2-(1,3-dimethoxypropan-2-yl)-1,2,3,4-tetrahydroisoquinolin-8-amine | C14 H22 N2 O2 | 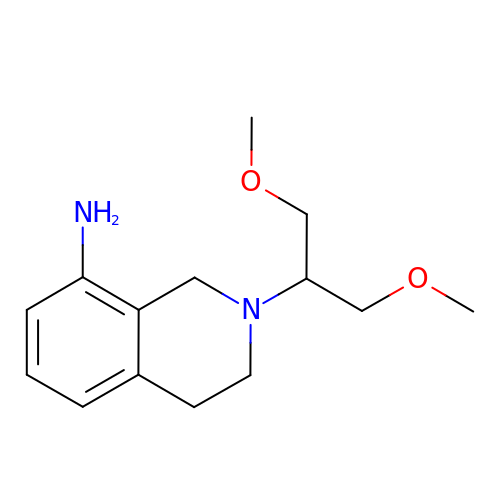NLRZZRKZNUFUOJ-UHFFFAOYSA-N>[2x]MAHHHHHHMAEFSIIDQYFNRQSHPDVALGIGDDSALITPPPNQQLVICADTLVAGRHFPLETSPHAIGWKSVAVNLSDIAAMGAKPHSILLAISLPQVDHEWLEGFSQGIYDCCNQFGVALIGGDTTQGPHLTITVTAMGWIETGKAVLRSGAKVGDYVCVSGQIGDAAYGLQHLGHSLQQRLDYPTPRCKLGEELKGLASSMIDVSDGLAQDLGHILKASKVGARLILEKLPVDPVLQQIEEQQRW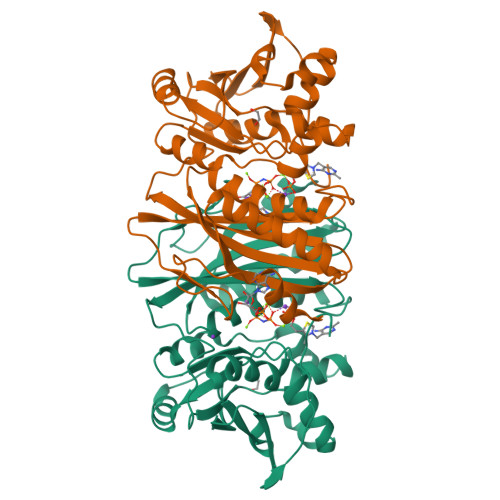QYALAGGDDYELCFTITPQNYEKLLQKQLDVKITMIGQIVEQTKLTFEHLGSDYPLQIHGYQHFAQQRW>UAUCAGUUAUAUGACUGACGGAACGUGGAAUUAACCACAUGAAGUAUAACGAUGACAAUGCCGACCG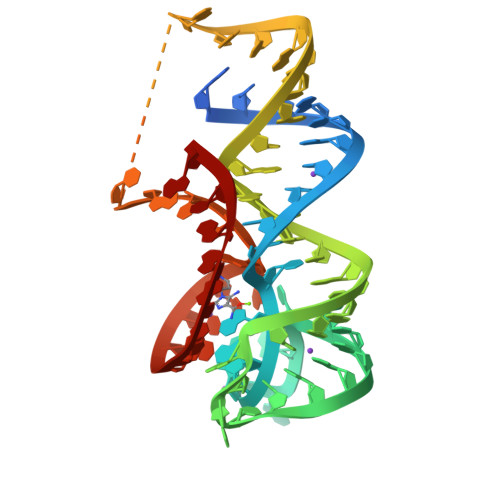UCUGGGCG[2x]>UUGCGUCGCGCCGGCGAAGUCG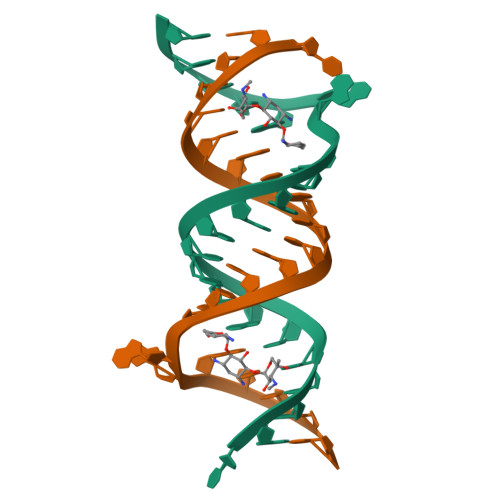C[2x]RBM45 is an RNA-binding protein with roles in neural development by regulating RNA splicing. Its dysfunction and aggregation are associated with neurodegenerative diseases such as amyotrophic lateral sclerosis (ALS) and frontotemporal lobar dementia (FTLD). RBM45 consists of three RNA-recognition motif (RRM) domains, two at the N-terminus (RRM1 and RRM2) and one at the C-terminus (RRM3), and a pseudo-RRM domain in the middle. In this work, we identified that the C-terminal RRM domain of human RBM45 (RBM45RRM3) sequence specifically binds GACG sequence RNA and solved the crystal structures of RBM45RRM3 in apo form and in complex with a single-stranded DNA that mimicked the recognized RNA.

To explore the RNA-recognition mechanism of RBM45RRM3, we attempted to co-crystallize RBM45RRM3 with RNA or ssDNA containing GACG sequence and finally solved the crystal structure of RBM45RRM3 in complex with an ssDNA 7-mer, 5′-GACGCAG-3′, at a resolution of 1.65 Å. There are also four RBM45RRM3 molecules per asymmetric unit, however, the space group and the packing pattern of the complex crystal are totally different from those of the protein-alone crystal. The final model includes the first six nucleotides of the ssDNA 7-mer, hereafter named from G1 to A6. The ssDNA binds to the positively charged β-sheet surface of RBM45 with its 5′ end bound to the β4 side and its 3′ end bound to the β2 side of the β-sheet, consistent with the conventional RNA binding pattern of RRMs. Superimposition with the protein-alone structure shows that the C-terminal loop of RBM45RRM3 in the complex structure is in a different direction. This loop is directly involved in the interaction with ssDNA, suggesting that the conformational change is most likely a result of ssDNA binding. Specifically, G1 binds to a hydrophobic patch formed by the side chains of Phe395 and Val397 in β1 and Met460 in β4; a γ-methyl of Val397 side chain contacts the purine ring of G1 via the CH–π interaction; the side-chain amino group of Lys458 in β4 forms hydrogen bonds with N7 and O6 of G1. The purine ring of A2 π–π stacks with the aromatic side chain of Phe395; the N1 and N3 of A2 form hydrogen bonds with the main-chain amino group of Asp463 in the C-terminal loop and the side-chain hydroxyl group of Tyr431 in β3, respectively; the N6 forms a hydrogen bond with the main-chain carbonyl group of Leu461 via a water molecule. The hydroxyl group of Tyr431 contacts the pyrimidine ring of C3 through OH–π interaction; two side-chain amino groups of Arg393 in β1 form hydrogen bonds with O2 and N3 of C3; the main-chain carbonyl group of Asp463 forms a hydrogen bond with N4 of C3. For G4, its purine ring π–π stacks with the side chain of Tyr422, whereas its N1 and N2 form two hydrogen bonds with the side-chain carboxyl group of Glu420 in β2 and its O6 forms a hydrogen bond with the side-chain amino group of Lys433 in β3.

>MQIQTDVVLPSCKKKAPAETPVKERLFIVFNPHPLPLDVLEDIFCRFGNLIEVYLVSGKNVGYAKYADRISANDAIATLHGKILNGVRLKVMLADSPREESNKRQRTYLEHHHHHH[4x]> 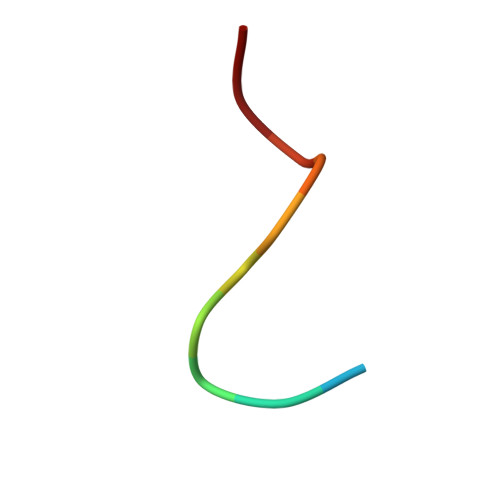SDDDMGFGLFD> MGRVEVRVEFEGDKMRVRLRNDSSTPVEVHIKVGDEKRTVTVNPGEEVEVTFSANDPHKFNRPQFTIEWGGGGRVEVRVEFEGDKMRVRLRNDSSTPVEVHIKVGDEKRTVTVNPGEEVEVTFSANDPHKFNRPQFTIEWG

Here, we devise geometrical principles for de novo designing single-chain immunoglobulin dimers, as a tunable two-domain architecture that optimizes biophysical properties through more favorable dimer interfaces. Here, we devise principles for de novo designing single-chain Ig dimers with interfaces diverging from Fvs, as a two-domain Ig architecture that is hard to find in nature and optimizes folding stability. We envisioned that de novo single-chain Ig dimers could be designed through two-layer edge-to-edge dimeric interfaces, resulting in extended Ig β-sandwiches. Key to such robustness is the two-layer edge-to-edge strand pairing at the interface between Ig domains, which involves a high number of backbone-backbone hydrogen bonds and protects oligomerization-prone β-sheet edges from solvent; overall favoring monomeric stability and solubility.

As the seventh (C-terminal) β-strand of each domain was found to be partly disordered and not present in the crystallographic dimer interface, we reasoned that the C-terminal region could be removed and then generated single-chain dimers of 6-stranded Ig monomers connected by a short β-hairpin loop; overall building a 12-stranded β-sandwich (right). To this aim, we removed the last nine residues of each domain, and designed a short loop connection (between 2 and 5 amino acids) between different anchoring residues (W68 or G69 of one monomer with G1 or R2 of the other monomer) by Rosetta fragment-based insertion. We found that the gap could be easily bridged with minimal backbone strain with loops of two or more residues connecting G69 with G1. The design with a two-residue hairpin loop (scIg12) was also found to have a strongly funneled energy landscape by Rosetta ab initio constrained folding simulations. We selected scIg12 for experimental characterization and, as the three scIg14 designs, was found to be well-expressed in E. coli, soluble, and monomeric by SEC-MALS. It had a far-UV circular dichroism spectra characteristic of all-β proteins and was stable at 95 °C or 7 M GdnCl. We succeeded in solving a crystal structure of scIg12 at 2.8 Å resolution by molecular replacement using the design model, and was found in excellent agreement with the computational model across the 12 β-strands (Cα-RMSD of 0.8 Å). A minor deviation was observed in the conformation of the designed connection. At the bottom, the designed linker is surrounded by a tightly packed area stabilized by aromatic stacking, and at the top it was found a cavity binding a glycerol molecule (as crystallization component) that is surrounded by the two β-arch helices (insets). The robustness of the scIg12 scaffold was borne out by nearly identical crystal structures obtained in the absence and presence of a 15-residue binding-loop insertion.> LENKPRIPVVWIHGLECTCCTESFIRSAHPLAKDVILSLISLDYDDTLMAAAGTQAEEVFEDIITQYNGKYILAVEGNPPLGEQGMFCISSGRPFIEKLKRAAAGASAIIAWGTCASWGCVQAARPNPTQATPIDKVITDKPIIKV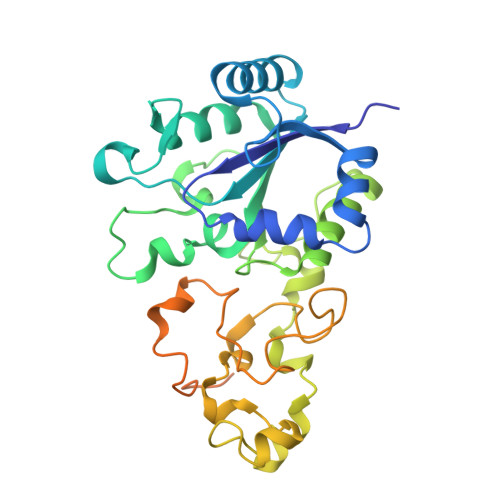PGCPPIPDVMSAIITYMVTFDRLPDVDRMGRPLMFYGQRIHDKCYRRAHFDAGEFVQSWDDDAARKGYCLYKMGCKGPTTYNACSSTRWNDGVSFPIQSGHGCLGCAENGFWDRGSFYSRVVDIPQMGTHSTADTVGLTALGVVAAAVGVHAVASAVDQRRRHNQQPTETEHQPGNEDKQA> GQELKGKYMKTPTGYLMVLRHGDNVLQNLEQLARDEHIPSASFVGIGFMSEATFGFYDFGRKQFDPKTYRNVEMANMTGSIAWKEGKPSIHAHGTVTDGTFQGAGGHLLGLTVGTGSCEITVTVYPQRLDRF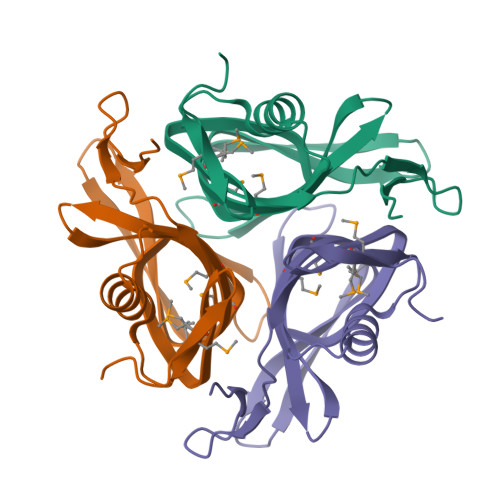VDPEIQANVLGLPQQ> QDGDAAKGEKEFNKCKACHMIQAPDGTDIIKGGKTGPNLYGVVGRKIASEEGFK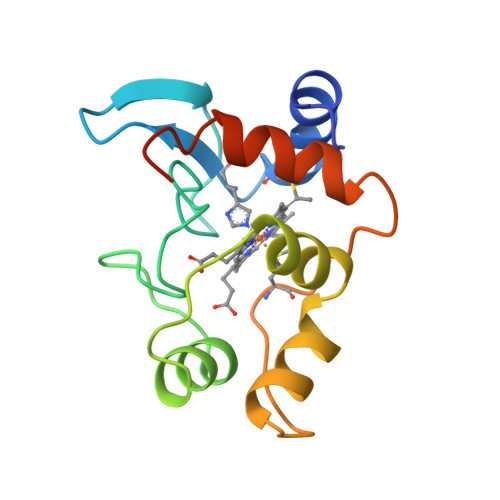YGEGILEVAEKNPDLTWTEADLIEYVTDPKPWLVKMTDDKGAKTKMTFKMGKNQADVVAFLAQNSPDAGGDGEAA> MSLPKPEDVLVAPNFGIQIDGVMVEYLNSVSNLQIEQDVIRYQQNQGTTGRNNVTLMPGVAKDGSVQVERGMSQSSVFTQWINDSMAGRMATARKNATIIVMDYEDNPVKRWNLRNAWCSKVVAGTLKAGDTNALTET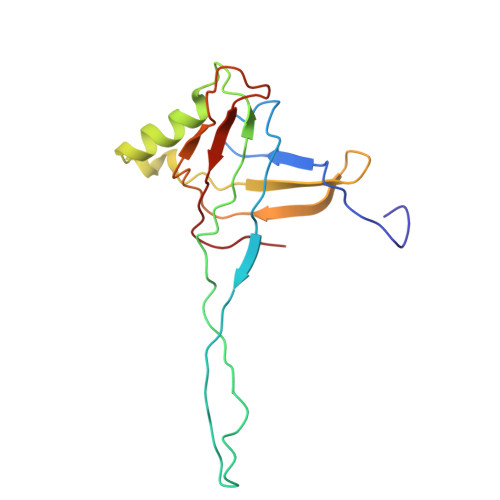ITIVFEELVVE>TETEQVDYGVTTPDG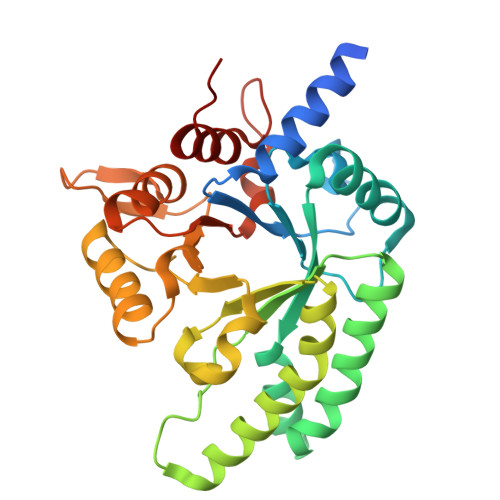QNPELYARYTQAVRNYKSRKHYAVCVRFDNGHSGDGEKDFLRSMPDSIDAVILENAATLNSADLEDIPVLQTNFATKVLFSFNLTSIKENAESSGQEIKTLLAPALEQMVSAITDNGLDGASISYTGDIGLGNNAAVNASITEMRQLLLDKITPLAKNGKIFFLESNPLFIPEANRDVFTRYVLNTTSSKNASQLRLLINEAIYYAGIPSDKLLITGDPELMTTDNNDGLVSQVPFFAIQVIDCGPIGGLMIQNVAADYSHANITYKETRGAIQTLNPSPLK[4x]> MTTDEGAKNNEESPTATVAEQGEDITSKKDRGVLKIVKRVGNGEETPMIGDKVYVHYKGKLSNGKKFDSSHDRNEPFVFSLGKGQVIKAWDIGVATMKRGEICH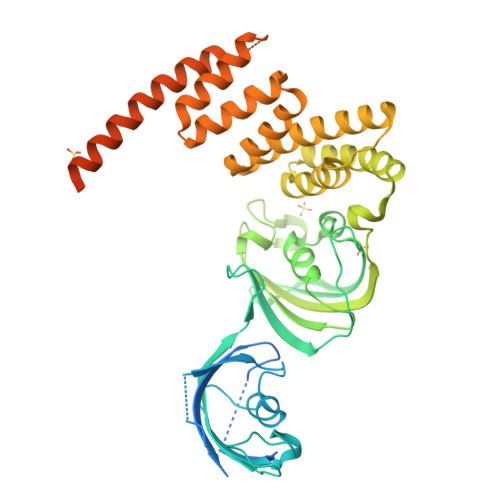LLCKPEYAYGSAGSLPKIPSNATLFFEIELLDFKGEDLFEDGGIIRRTKRKGEGYSNPNEGATVEIHLEGRCGGRMFDCRDVAFTVGEGEDHDIPIGIDKALEKMQREEQCILYLGPRYGFGEAGKPKFGIEPNAELIYEVTLKSFEKAKESWEMDTKEKLEQAAIVKEKGTVYFKGGKYMQAVIQYGKIVSWLEMEYGLSEKESKASESFLLAAFLNLAMCYLKLREYTKAVECCDKALGLDSANEKGLYRRGEAQLLMNEFESAKGDFEKVLEVNPQNKAARLQISMCQKKAKEHNERDRRIYANMFKKFAEQDAKEEANKAMGKKTSEGVTNEKGTDSQAMEEEKPEGHV> X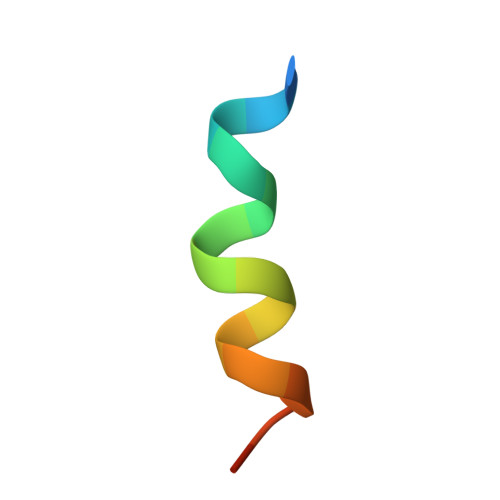PWWECLSQADDCDFRX> GSGKWVIDPSELTFVQEIGSGQFGLVHLGYWLNKDKVAIKTIREGAMSEEDFIEEAEVMMKLSHPKLVQLYGVCLEQAPICLVFEFMEHGCLSDYLRTQRGLFAAETLLGMCLDVCEGMAYLEEACVIHRDLAARNCLVGENQVIKVSDFGMTRFVLDDQYTSSTGTKFPVKWASPEVFSFSRYSSKSDVWSFGVLMWEVFSEGKIPYENRSNSEVVEDISTGFRLYKPRLASTHV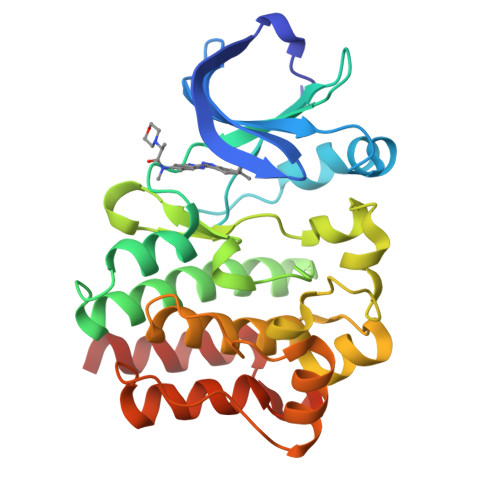YQIMNHCWRERPEDRPAFSRLLRQLAEIAESGL> MKAVLFDIDGTILTEEPLIMLFLPQVYDKLSRKLGISK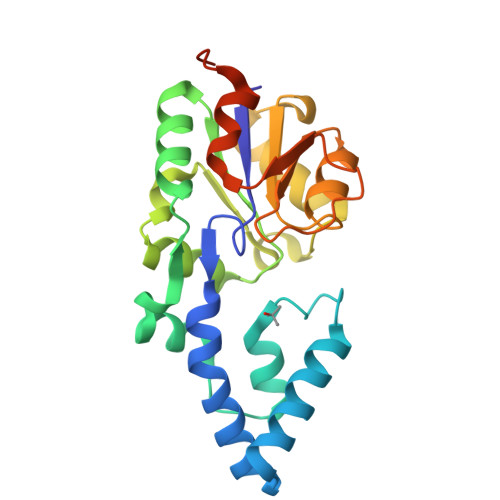DEARERFLSEILGRRDSYDWHDWNFFFKLFDLDLKYEELLERYPHKLQVYPDTIPTLEWLRDTGYKLGIVTSGPKYQRLKLKLTGLLDYFDVVITRDDVNAIKPEPKIFLYTIERLGVEPGEAVMVGDSLSQDVYGAKSVGMTAVWINRNGDRGYNMADYEIRTLYELRKILGGERVDKLAAALEHHHHHH>[2x]MSLSKKIAVIGECMIELSEKGADVKRGFGGDTLNTSVYIARQVDPAALTVHYVTALGTDSFSQQMLDAWHGENVDTSLTQRMENRLPGLYYIETDSTGERTFYYWRNEAAAKFWLASEQSAAICEELANFDYLYLSGISLAILSPTSREKLLSLLRECRAKGGKVIFDNNYRPRLWASKEETQQVYQQMLECTDIAFLTLDDEDALWGQQPVE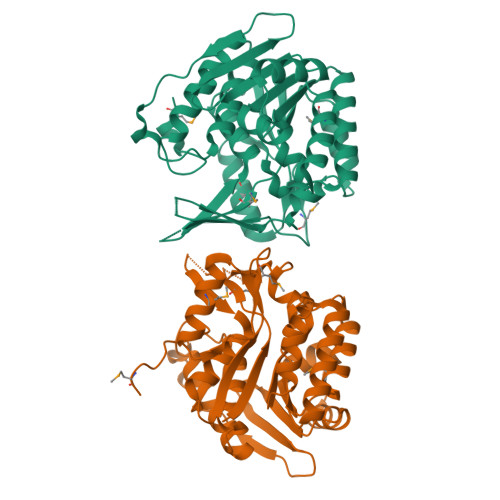DVIARTHNAGVKEVVVKRGADSCLVSIAGEALVDVPAVKLPKEKVIDTTAAGDSFSAGYLAVRLTGGSAENAAKRGHLTASTVIQYRGAIIPREAMPAEGHHHHHH> GSQNQERLCAFKDPYQQDLGIGESRISHENGTILCSKGSTCYGLWEKSKGDINLVKQGCWSHIGDPQECHYEECVVTTTPPSIQNGTYRFCCCSTDLCNVNFTENFPPPD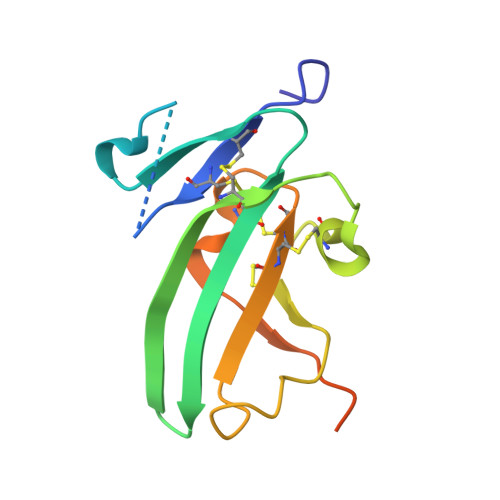TTPLSPPHSFNRDET> MEEVKKKLEEVWKKAKEDAGDNEKFLELLELILENPEILEILELYVFINKEDVVEKLFDVIKKAVEDAGDNEKFLELLKEMLSNPEIFEILLEYVYIKKEDVVEKLFEVIKQAVEDAGDNPVFLKLLKKMISNPEIFEILLEYVYIGKEE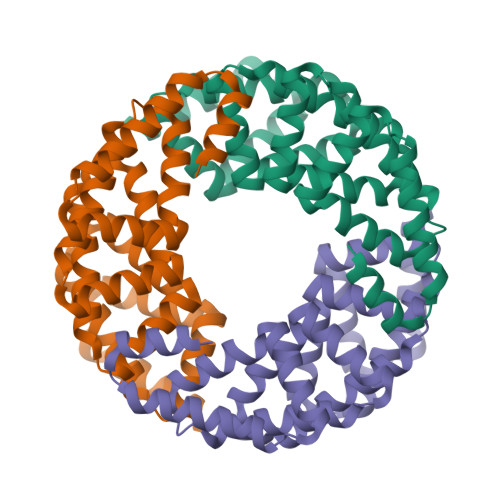VVKKFFEVIKQAVEDAGNNPIFLKLLEKIILDPERFKKLLEKVEVGEEEEVKAEFKEIKKAVEEAGNDPIKLKELEEKLGSWLEHHHHHH> ALQTIINARLPGEEGLWQIHLQDGKISAIDAQSGVMPITENSLDAEQGLVIPPFVEPHIHLDTTQTAGQPNWNQSGTLFEGIERWAERKALLTHDDVKQRAWQTLKWQIANGIQHVRTHVDVSDATLTALKAMLEVKQEVAPWIDLQIAAFPQEGILSYPNGEALLEEALRLGADVVGAIPHFEFTREYGVESLHKTFALAQKYDRLIDVHCDEIDDEQSRFVETVAALAHHEGMGARVTASHTTAMHSYNGAYTSRLFRLLKMSGINFVANPLVNIHLQGRFDTYPKRRGITRVKEMLESGINVCFGHDDVCGPWYPLGTANMLQVLHMGLHVCQLMGYGQINDGLNLITHHSARTLNLQDYGIAAGNSANLIILPAENGFDALRRQVPVRY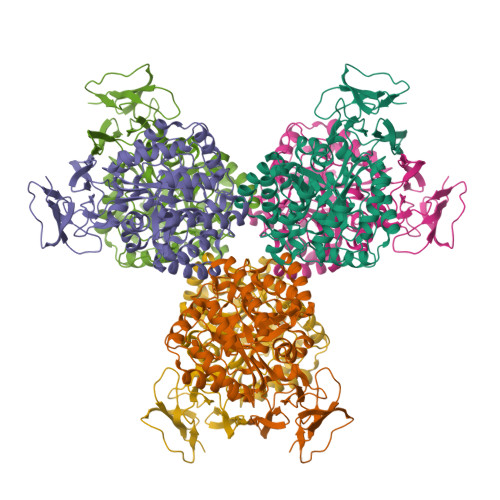SVRGGKVIASTQPAQTTVYLEQPEAIDYKR> NKFVEQDDWFHDRRVYLDALENQLKALL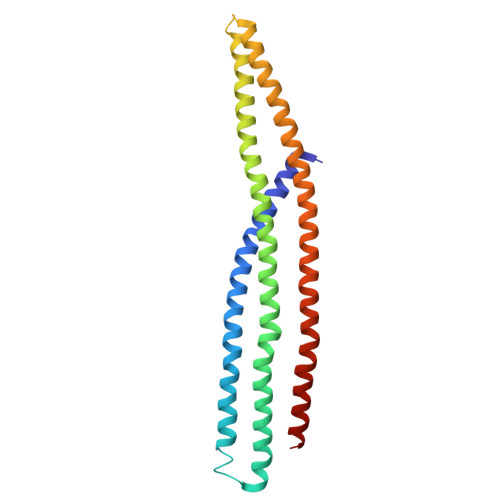KAMDNMVAQRKAMAEAAADFSASLHALSTVELSPTLSGPLDALSELQLAIRDVYERQAQQDVLTFGIIIEEYIRLIGSVKQAFSQRQKAFHSWHSAESELMKKKAAQDKLLRQGKTQQDRLNQVNAEVIDAERKVHQARLLFEDMGRLLRSELDRFEREKVEDFKSGVETFLESAVEAQKELIEKWETFLMQ>METDNVELAQSKRKVVLAEQGSFYIGGRTVTGPGKFDPSKPVIPYSNEGATFYINQMYVNFQAPVRPRGLPLVFWHGGGLTGHIWESTPDGRPGFQTLFVQDRHTVYTIDQPGRGRGNIPTFNGPFGQLEEESIVNTVTGNSSKEGAWVRDRLGPAPGQFFENSQFPRGYEDNYFKEMGFSPSISSDEIVDAVVKLVTHIGPCVLVTHSASGVLGMRVATHAKNVRGIVAYEPATSIFPKGKVPEIPPLADKKSQIFPPFEIQESYFKKLAKIPIQFVFGDNIPKNPKSAYWFLDWWRVTRYAHSLSLEAINKLGGQASLLDLPTAGLRGNTHFPFTDRNNVQVASLLSDFLGKHGLDQNESLEHHHHHH[4x]

SulE, an esterase, which detoxifies a variety of sulfonylurea herbicides through de-esterification, provides an attractive approach to remove environmental sulfonylurea herbicides and develop herbicide-tolerant crops. SulE catalyzes the de-esterification of a variety of sulfonylurea herbicides, such as MM, BM, SM, TM, TrM, EM, and CE, to the corresponding herbicidal-inactive parent acid. The structures show that SulE is a dimer with a lid loop in a domain-swapped β-hairpin covering the active site from the opposing monomer. SulE shows a similar catalytic triad consisting of Ser209, His333, and Glu232 at its active site.

To elucidate the catalytic mechanism of SulE, we solved the crystal structures of wild-type SulE in complex with CA, mutant S209A in complex with MM, and mutant S209A/H333A in complex with MM, SM, TM, TrM, EM, BM, and CE in the range of 1.29–1.63 Å. The overall fold of these structures is similar to that of the apo form, with rmsd values in the range of 0.1–0.2 Å after the superimposition of all Cα atoms. The SulE-CA complex structure represents the binding of the enzyme to the product. Structural comparison showed that CA and CE are well superimposed at the active site, indicating that the substrate and product bind to SulE using the same set of interactions. A water molecule Wat719 was observed near His333. Wat719 formed hydrogen bonds with His333 and the carboxyl oxygen atom of CA, presumably the deacylating water molecule. However, in SulE, the binding of product and substrate at the active site was similar, and no significant product inhibition was observed.2'-C-methyl-5'-O-({5-[(3aS,4S,6aR)-2-oxohexahydro-1H-thieno[3,4-d]imidazol-4-yl]pentanoyl}sulfamoyl)adenosine 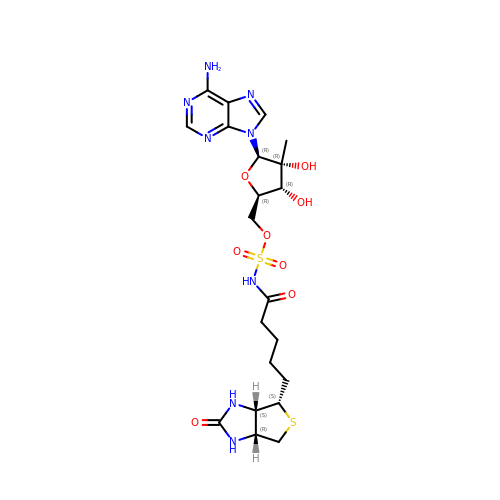| C21 H30 N8 O8 S2 | BGUXFAITPCEERX-BKJQVYKZSA-N>[3x]MSSKPKPIEIIGAPFSKGQPRGGVEKGPAALRKAGLVEKLKETEYNVRDHGDLAFVDVPNDSPFQIVKNPRSVGKANEQLAAVVAETQKNGT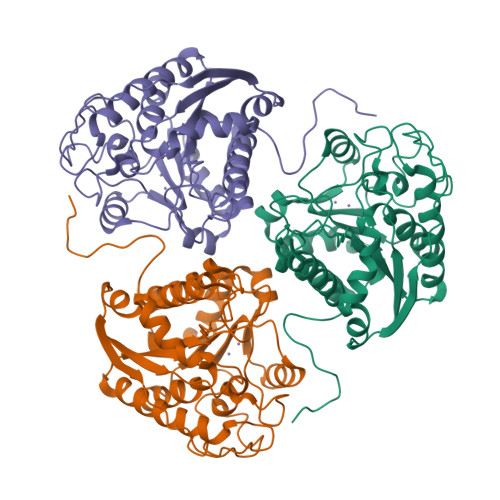ISVVLGGDHSMAIGSISGHARVHPDLCVIWVDAHTDINTPLTTSSGNLHGQPVAFLLKELKGKFPDVPGFSWVTPCISAKDIVYIGLRDVDPGEHYIIKTLGIKYFSMTEVDKLGIGKVMEETFSYLLGRKKRPIHLSFDVDGLDPVFTPATGTPVVGGLSYREGLYITEEIYKTGLLSGLDIMEVNPTLGKTPEEVTRTVNTAVALTLSCFGTKKEGNHKPETDYLKPPK>[4x]MKILKLQTLRGPNYWSIHRHKLVVMRLDLEDLYEKYTSDIPGFYKGLTEVLPSLVEHLCSPGVKGGFLTRVEKGTLIGHVIEHVAIELQELAGMPVGFGRTRETSTTGVFQVVIEYENEQAGRYAARAAVRLCQSIVDTGTYPATELQQDLEDLKELKNQASLGPSTEAIVKEAEARGIPWTQLGARFMIQFGYGVNQKKIQATLSNQTGILGVELACDKEGTKRILKDAGVPVPRGTVARYFDELQDAIEYVGGYPIVIKPLDGNHGRGITIDVKNWQEAEEAYDLARKASKTKTVIVERYYTGKDHRVLVVNGKVVAVAERVPAHVVGNGKSTIAELIEETNRDPQRGDGHDNILTRITVDKSALDILGKQGYSIDSIPLKGKKCFLRATANLSTGGIAVDRTDEIHPENVWLLSRVAKIIGLDIAGIDVVTEDISQPLREVEGVIVEVNAAPGFRMHVAPSRGLARNVAGAVMDMLFP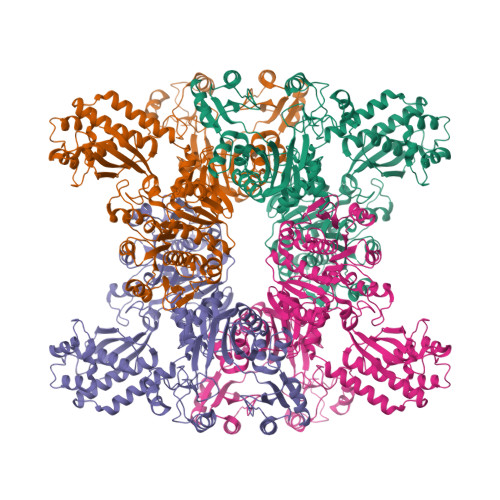GSKNGRIPILSVTGTNGKTTTTRLLAHIIKQTGKVVGYTTTDGTYIGEYLAETGDNTGPQSAHLILSDPTVEVAVLETARGGILRSGLGFSSCEVGIVLNVTADHLGIGDIDTIEQLAKLKSVVAESVMPKGYAVLNAEDPLVAAMADRVKGQVAYFSMDPNNELLLRHTEAGGLAAIYENGYISILKGDWTLRIEKAVNVPITMAGKAPFMIANALAACLAVFTQGVKIEHIRKGLSTFVASVDQTPGRMNMFNMGSYHALVDYAHNPASYEALGGFVRNWPGKRIGVVGGPGDRRDEDFVSLGELAADIFDEIIIKEDDDTRGRPRGNAAELICQGVKQFLNGIKNSESKATYESILDETAAINTALDRAPIDGLVVILPESVNRAISLIEGRHVIQDIELLQDSQREPKDQEVLKSSILEHHHHHH>MTNIRVAIVGYGNLGRSVEKLIAKQPDMDLVGIFSRRATLDTKTPVFDVADVDKHADDVDVLFLCMGSATDIPEQAPKFAQFACTVDTYDNHRDIPRHRQVMNEAATAAGNVALVSTGWDPGMFSINRVYAAAVLAEHQQHTFWGPGLSQGHSDALRRIPGVQKAVQYTLPSEDALEKARRGEAGDLTGKQTHKRQCFVVADAADHERIENDIRTMPDYFVGYEVEVNFIDEATFDSEHTGM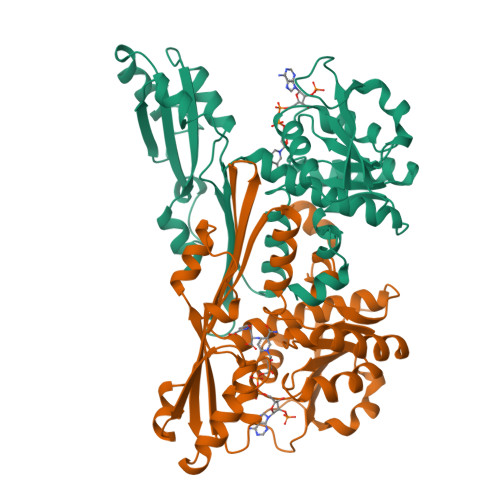PHGGHVITTGDTGGFNHTVEYILKLDRNPDFTASSQIAFGRAAHRMKQQGQSGAFTVLEVAPYLLSPENLDDLIARDV[2x]Thioredoxins (Trxs) are ubiquitous enzymes that regulate the redox state in cells. In Drosophila, there are two germline-specific Trxs, Deadhead (Dhd) and thioredoxin T (TrxT), that belong to the lethal(3)malignant brain tumor signature genes and to the ‘survival network’ of genes that mediate the cellular response to DNA damage. Trxs share a conserved catalytic motif, with two conserved cysteine residues embedded in a canonical fold consisting of five β-strands and four α-helices. Drosophila Dhd, TrxT and Trx-2 (previously determined; Wahl et al., 2005) are intermediate between these two characteristic folds, displaying four α-helices (as in all Trx structures) but only four β-strands (β2–β5).

TrxT is testis-specific and associates with the lampbrush loops of the Y chromosome. The second difference is related to the TrxT fold, which is composed of a highly conserved core and a variable C-terminal domain, with the latter being absent in most canonical Trxs. This extra domain is mostly unstructured, with a high ratio of negatively charged residues. In D. melanogaster, this C-terminal domain is attached to the protein core via a covalent link that stabilizes a closed conformation that partially covers the catalytic site. The regions connecting Gly107 to Asp111 and His120 to Cys125 were also traceable, but unfortunately the fragment connecting Asp111 to His120 and the last 26 amino acids were not visible in the density, which is also in agreement with the rapid motions and negative 15N–[1H] NOE values measured for these residues. Moreover, in the case of TrxT the crystals contain two TrxT molecules engaged with a symmetry-related neighbor stabilized through the coordination of a Zn atom (which was present in the crystallization condition). The zinc is bound between Asp65 and Glu69 from monomer A and His105 and Glu88 from monomer B [Supplementary Fig. S3(b)]. Overall, these results underline the hypothesis that the C-terminal domain shields the active site of TrxT and modulates its redox activity.

> MVYPVRNKDDLDQQLILAEDKLVVIDFYADWCGPCKIIAPKLDELAHEYSDRVVVLKVNVDENEDITVEYNVNSMPTFVFIKGGNVLELFVGCNSDKLAKLMEKHAGVYTDEAADVKAVHIDGECIVDLTAESSESDNDNNNVNEVSAHDENAVLEH>GSMPPQLHNGLDFSAKVIQGSLDSLPQEVRKFVEGNAQLCQPEYIHICDGSEEEYGRLLAHMQEEGVIRKLKKYDNCWLALTDPRDVARIESKTVIITQEQRDTVPIPKSGQSQLGRWMSEEDFEKAFNARFPGCMKGRTMYVIPFSMGPLGSPLAKIGIELTDSPYVVASMRIMTRMGTSVLEALGDGEFIKCLHSVGCPLPLKKPLVNNWACNPELTLIAHLPDRREIISFGSGYGGNSLLGKKCFALRIASRLAKEEGWLAEHMLILGITNPEGKKKYLAAAFPSACGKTNLAMMNPTLPGWKVECVGDDIAWMKFDAQGNLRAINPENGFFGVAPGTSVKTNPNAIKTIQKNTIFTNVAETSDGGVYWEGIDEPLAPGVTITSWKNKEWRPQDEEPCAHP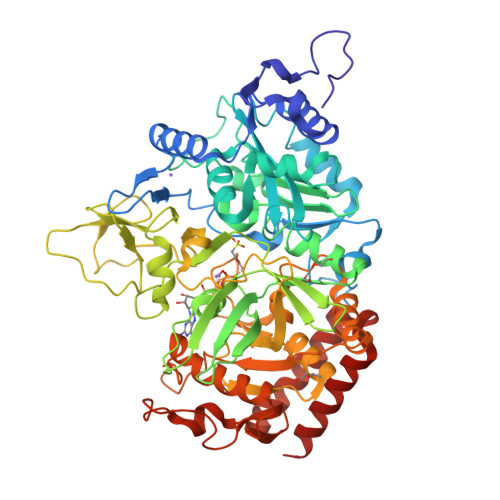NSRFCTPASQCPIIDPAWESPEGVPIEGIIFGGRRPAGVPLVYEALSWQHGVFVGAAMRSEATAAAEHKGKVIMHDPFAMRPFFGYNFGKYLAHWLSMAHRPAAKLPKIFHVNWFRKDKNGKFLWPGFGENSRVLEWMFGRIEGEDSAKLTPIGYVPKEDALNLKGLGDVNVEELFGISKEFWEKEVEEIDKYLEDQVNADLPYEIERELRALKQRISQM[2x]> KMGLLVMAYGT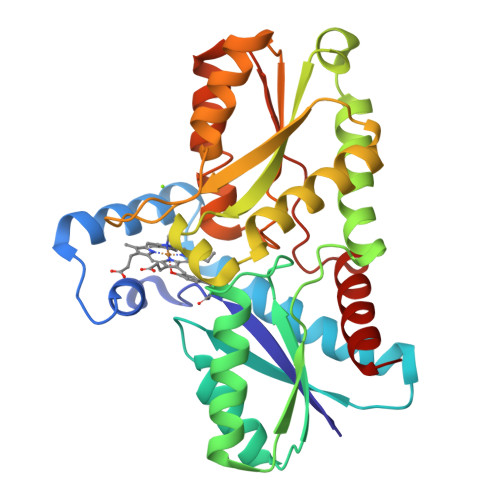PYKEEDIERYYTHIRRGRKPEPEMLQDLKDRYEAIGGISPLAQITEQQAHNLEQHLNEIQDEITFKAYIGLKHIEPFIEDAVAEMHKDGITEAVSIVLAPHFSTFSVQSYNKRAKEEAEKLGGLTITSVESWYDEPKFVTYWVDRVKETYASMPEDERENAMLIVSAHSLPEKIKEFGDPYPDQLHESAKLIAEGAGVSEYAVGWQSEGNTPDPWLGPDVQDLTRDLFEQKGYQAFVYVPVGFVADHLEVLYDNDYECKVVTDDIGASYYRPEMPNAKPEFIDALATVVLKKLGR> SNAMSPSPLISHRAASADLAGMVRQARQRILLQGNVPGFDVARQIELLHGLAESELGRFLLLYRGLNAEWTHRLVTHQPGSGALAPLERVFYERLPAVLATRERHGHFRRALQRHLRPGCVVASVPCGWMSELLALDYSACPGVQLVGIDYDPEALDGATRLAAGHALAGQITLHRQDAWKLDTREGYDLLTSNGLNIYEPDDARVTELYRRFWQALKPGGALVT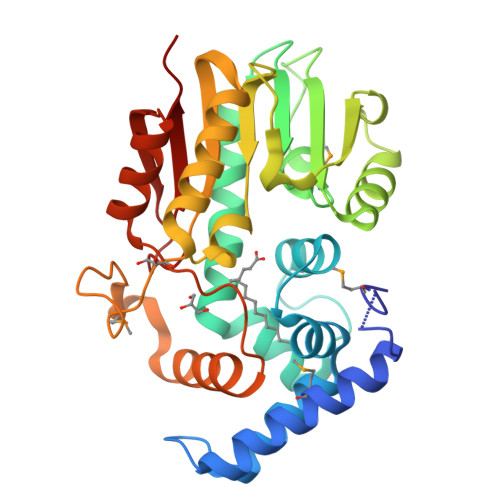SFLTPPPALSPDSPWDMQAIDPHDLQLQQLVFTRLIQPRWNALRTHAQTRAQLEEAGFTDLRFEDDRARLFPTVIARKPA> AAHHHHHHSSGLVPRGSHMANKAVNDFILAMNYDKKKLLTHQGESIENRFIKEGNQLPDEFVVIERKKRSLSTNTSDISVTATNDSRLYPGALLVVDETLLENNPTLLAVDRAPMTYSIDLPGLASSDSFLQVEDPSNSSVRGAVNDLLAKWHQDYGQVNNVPMQYEKITAHSMEQLKVKFGSDFEKTGNSLDIDFNSVHSGEKQIQIVNFKQIYYTVSVDAVKNPGDVFQDTVTVEDLKQRGISAERPLVYISSVAYGRQVYLKLETTSKSDEVEAAFEALIKGVKVAPQTEWKQILDNTEVKAVILGGDPSSGARVVTGKVDMVEDLIQEGSRFTADHPGLPISYTTSFLRDNVVATFQNSTDYVETKVTAYRNGDLLLDHSGAYVAQYYITWDELSYDHQGKEVLTPKAWDRNGQDLTAHFTTSIPLKGNVRNLSVKIRECTGLAWEWWRTVYEKTDLPLVRKRTISIWGTTLYPQVEDKVENA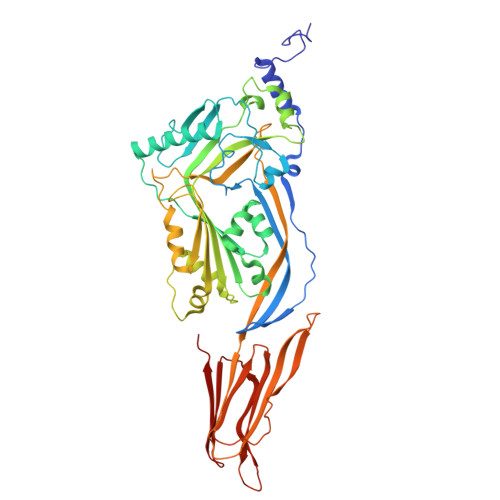A We have solved the crystal structures of the MyoVa globular tail domain in complex with Spir-2-GTBM and in complex with Rab11. The MyoV-GTD is composed of two closely apposed subdomains (SD-1 and SD-2). We have also shown that the MyoV-GTD links Spir-2 and Rab11 into a tripartite complex in vitro and in cells. The Spir:MyoV interaction contributes to the motor activation and to the coordination of the specific membrane recruitment of both actin polymerization and motor machineries required for force production powered by MyoV.

A search for the mechanism that controls the targeting of the Spir:FMN complex to Rab11:MyoV vesicles revealed a conserved MyoV globular tail domain binding motif (GTBM) in Spir proteins that mediates a direct interaction between Spir and MyoV. We further characterized the Spir:MyoVa binding by solving a crystal structure of the complex, which allowed us to identify the protein interaction sites and depict the stabilizing interactions within the complex at atomic detail. The Spir-2-GTBM peptide binds to the SD-1 of the MyoVa-GTD in an extended conformation, forming a two-turn alpha helix at the end, in the cleft between helices H3 and H5. Spir-2-GTBM can be accommodated on the surface of MyoVa without conformational changes in the GTD, and the Spir-GTBM binding pocket is structurally conserved in MyoVb and MyoVc. The Spir-2 and MLPH GTBMs exhibit some sequence similarity and comparison of the complex structures shows that their N-terminal regions interact with MyoVa in a very similar way, forming a network of hydrogen bonds with the H4’’-H5-loop and similarly positioning two conserved leucine residues of the motif (L408 and L409 in Spir-2; L188 and L189 in MLPH) within cavities of the MyoVa-GTD surface. Mutation of the two highly conserved Spir leucine residues to alanines significantly impairs Spir-2 binding to MyoV. The Spir-GTBM C-terminal part anchors itself in the MyoVa hydrophobic cleft between helices H3 and H5 using L414 and M417 side chains; and the small side chain of the strictly conserved Ala411 binds in proximity to the MyoVa Tyr1596 side chain. Interestingly, the MyoV-GTD Spir-2 binding site partially overlaps with that of melanophilin (MLPH). The Spir-GTBM interacts with the same binding pocket in the MyoV-GTD SD-1 that can also be occupied by a short N-terminal linker preceding the MyoV-GTD implicated in stabilizing the OFF state of the myosin. Binding of the Spir-GTBM would displace the N-terminal linker and contribute to MyoV activation.

> GAMGSVNIPRKEKDFQGMLEYKKEDEQKLVKNLILELKPRGVAVNLIPGLPAYILFMCVRHADYLNDDQKVRSLLTSTINSIKKVLKKRGDDFETVSFWLSNTCRFLHCLKQYSGEEGFMKHNTSRQNEHCLTNFDLAEYRQVLSDLAIQIYQQLVRVLENILQPMIVSGMLEHETIQGVSGVKPTGLRKRTSSIADEGTYTLDSILRQLNSFHSVMCQHGMDPELIKQVVKQMFYIIGAITLNNLLLRKDMCSWSKGMQIRYNVSQLEEWLRDKNLMNSGAKETLEPLIQAAQLLQVKKKTDDDAEAICSMCNALTTAQIVKVLNLYTPVNEFEERVSVSFIRTIQMRLRDRKDSPQLLMDAKHIFPVTFPFNPSSLALETIQIPASLGLGFISRV;> QRPRPRVLLKAPTLAEMEEMNTSEEEE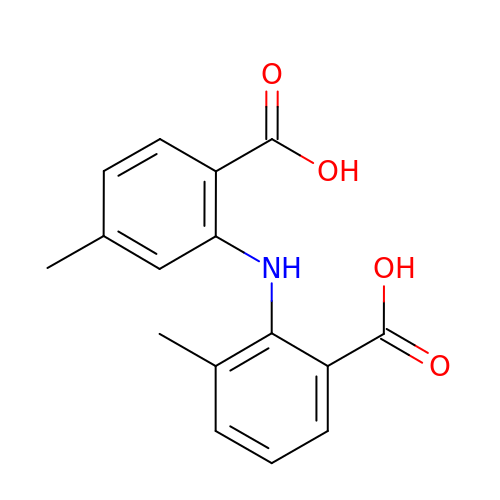2-[(2-carboxy-5-methylphenyl)amino]-3-methylbenzoic acid | C16 H15 N O4 | AQDGEUMMMQRBPR-UHFFFAOYSA-N> GTIITVTAQANEKNTRTVSTAKGDKKIISVPLFEKEKGSNVKVAYGSAFMPDFIQMGDTVTVSGRVQAKESGEYVNYNFVFPTVEKVFITNDNSSQSQAKQDLFG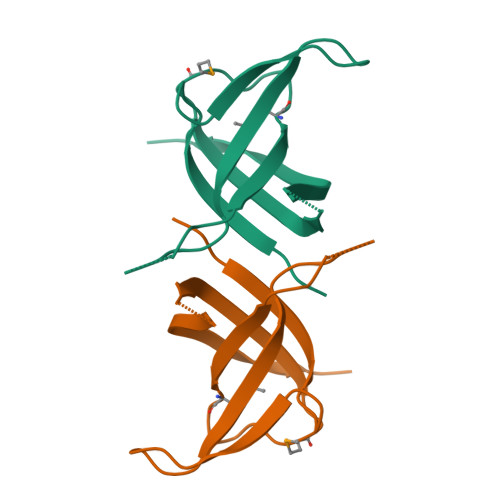GSEPIEVNSEDLPF>[2x]MATSLNTIDIQGDILVGMHKQKQLFYFFAINDPATFKTHLASDIAPVVASVTQLSNVATQPLVALNIAFSNTGLLALGVTDNLGDSLFANGQAKDATSFKESTSSWVPQFAGTGIHGVIILASDTTDLIDQQVASIESTFGSSISKLYSLSASIRPGNEAGHEM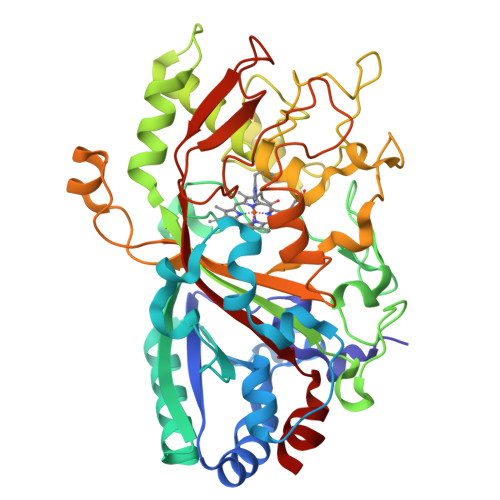FGFLDGIAQPAINGFNTPLPGQNIVDAGVIITGATNDPITRPSWAVGGSFLAFRQLEQLVPEFNKYLLDNAPAGSGSLQARADLLGARMVGRWKSGAPIDLTPTADDPALGADAQRNNNFTYSHAGFDLGSDQSHCPFSAHIRKTRPRADLGGSLTPPNLSAGANSIMRSGIPYGPEVTSAESASNTTTQERGLAFVAYQAQLSQGFHFLQQTSADNANFPPGKTPATVGLDPIIGQNNGQPRVVNGLLPSNSSASLSIPQFVVSHGGEYFFSPPISAIGGRLSA> MIVKKKLAAGEFAETFKNGNNITIIKAVGELVLRAYGADGGEGLRTIVRQGVSIKGMNYTSVMLHTEYAQEIEYWVGDLDYSFQEQTTKS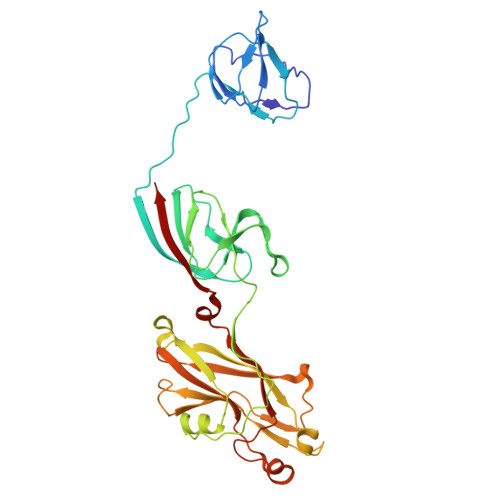RDVNSFQIPLRDGVRELLPEDASRNRASIKSPVDIWIGGENMTALNGIVDGGRKFEAGQEFQINTFGSVNYWVSDEEIRVFKEYSARAKYAQNEGRTALEANNVPFFDIDVPPELDGVPFSLKARVRHKSKGVDGLGDYTSISVKPAFYITEGDETTDTLIKYTSYGSTGSHSGYDFDDNTLDVMVTLSAGVHRVFPVETELDYDAVQEVQHDWYDESFTTFIEVYSDDPLLTVKGYAQILMERT>MKTIIINGVQFNTDEDTTILKFARDNNIDISALCF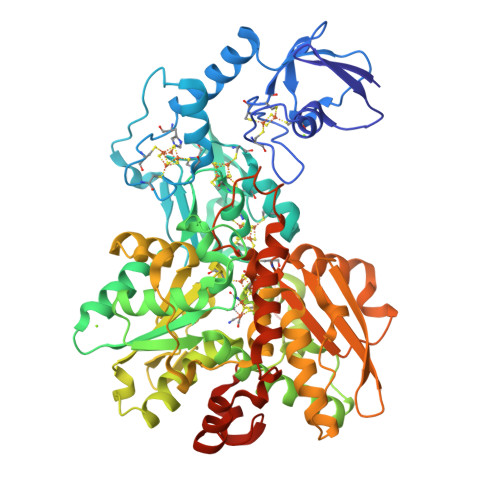LNNCNNDINKCEICTVEVEGTGLVTACDTLIEDGMIINTNSDAVNEKIKSRISQLLDIHEFKCGPCNRRENCEFLKLVIKYKARASKPFLPKDKTEYVDERSKSLTVDRTKCLLCGRCVNACGKNTETYAMKFLNKNGKTIIGAEDEKCFDDTNCLLCGQCIIACPVAALSEKSHMDRVKNALNAPEKHVIVAMAPSVRASIGELFNMGFGVDVTGKIYTALRQLGFDKIFDINFGADMTIMEEATQLVQRIENNGPFPMFTSCCPGWVRQAENYYPELLNNLSSAKSPQQIFGTASKTYYPSISGLDPKNVFTVTVMPCTSKKFEADRPQMEKDGLRDIDAVITTRELAKMIKDAKIPFAKLEDSEADPAMGEYSGAGAIFGATGGVMEAALRSAKDFAENAELEDIEYKQVRGLNGIKEAEVEINNNKYNVAVINGASNLFKFMKSGMINEKQYHFIEVMACHGGCVNGGGQPHVNPKDLEKVDIKKVRASVLYNQDEHLSKRKSHENTALVKMYQNYFGKPGEGRAHEILHFKYKKSAWSHPQFEK[2x]> RLETGNTVADISLGLINFLYSNFVPGGGFIVGLLELIWGFIGPSQWDIFLAQIEQLISQRIEEFARNQAISRLEGLSNLYKCYVRAFSDWEKDPTNPALRECMRIQFNDMNSALITAIPLFRVQNYEVALLSVYVQAANLHLSILRDVSVFGERWGYDTATINNRYSDLTSLIHVYTNHCVDTYNQGLRRLEGRFLSDWIVYNRFRRQLTISVLDIVAFFPNYDIRTYPIQTATQLTREVYLDLPFINENLSPAAVYPTFSAAESAIIRSPHLVDFLNSFTIYTDSLARSAYWGGHLVNSFRTGTTTNLIRSPLYGREGNTERPVTITASPSVPIFRTLSYPTGLDNSNPVAGIEGVEFQNTISRSIYRKSGPIDSFSELPPQDASVSPAIGYSHRLCHATFLERISGPRIAGTVFSWTHRSASPTNEVSPSRITQIPWVKAHTLASGA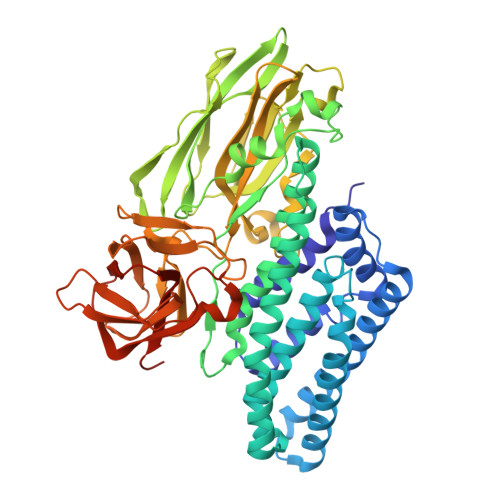SVIKGPGFTGGDILTRNSMGELGTLRVTFTGRLPQSYYIRFRYASVANRSGTFRYSQPPSYGISFPKTMDAGEPLTSRSFAHTTLFTPITFSRAQEEFDLYIQSGVYIDRIEFIPVTATFEAEYDLER>MSYMNFDPKPLGDTNIFKPIKIGNNELKHRVVMPALTRMRAIAPGNIPNTEWAEEYYRQRSQYPGTLIITEGTFPSAQSGGYPNVPGIWSKEQLAEWKKIFNAIHENKSFVWVQLWVLGRQAWPEVLKKEGLRYDSATDDLYMGEEEKERALKANNPQHGITKEEIKQYIKEYVDAAKKAIDAGADGVQIHSANGYLLNQFLDPISNNRTDEYGGSIENRARFTLEVVDAVVDAVGAERTSIRFSPYGTFGTMSGG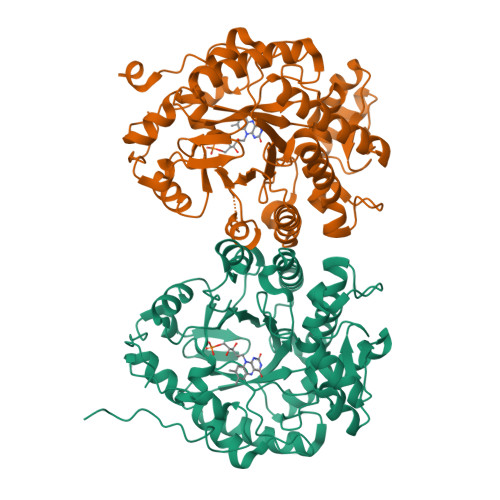ENPGIVAQYAYVIGELEKRARAGKRLAFIDLVEPRVTDPFLPEFEKWFKEGTNEFIYSIWKGPVLRVGNYALDPDQATLDSKKPNTLIGYGRSFIANPDLVYRLEKGLPLNKYDRNTFYTFTKEGYTDYPSYEESVAKGYKKEEKKY[4x]>[2x]GAMGFNKILVVCVGNICRSPTGERVLQKLLPNKTVASAGIAAEKSRLIGKPADAMAIEVAKENCVDVENHQSQQLTSALCSQYDLILVMEKGHMEALTQIAPEARGKTMLFGQWIGQKDIPDPYRQSKEAFVHAYQLIDEAAQAWAKKL

Protein tyrosine phosphorylation regulates the production of capsular polysaccharide, an essential virulence factor of the deadly pathogen Vibrio vulnificus. The process requires the protein tyrosine kinase Wzc and its cognate phosphatase Wzb, both of which are largely uncharacterized. VvWzb belongs to the low-molecular-weight protein tyrosine phosphatase (LMWPTP) family. Interestingly, it contains an extra four-residue insertion in the W-loop, distinct from all known LMWPTPs.

VvWzb crystallized in the space group P212121, with two protein molecules in one asymmetric unit. The two molecules formed a dimer in the crystal, with an interface area of about 900 Å2. However, this seems to be a crystallographic dimer, since VvWzb existed as a monomer in solution, indicated by gel filtration. VvWzb adopts a typical LMWPTP α/β fold. Like other LMWPTPs, the active site crevice of free VvWzb is composed of the P-loop (residues Cys9−Ser16), D-loop (residues Lys115−Gln123), and W-loop (residues Ile37−Lys47). The W-loop of VvWzb, which is longer than any known LMWPTP by harboring a four-residue insert (40EKSR43), bulges out, with residues Ser42, Arg43, and Leu44 located at the tip region and residue Glu40 pointing toward the active site. Compared with the D-loop wall, which is relatively orthogonal to the P-loop bottom, the W-loop wall seems to be laid flat. In such a configuration, the active site crevice of free VvWzb is wide and shallow, being readily accessible for the substrate. Due to the presence of Glu40, the W-loop wall region of the crevice is negatively charged. In the absence of ligand, the supposed phosphate-binding site is occupied by a chloride ion and a few water molecules; they interact with the P- and D-loop residues via extensive hydrogen bonding.2-(pyridin-2-yl)pyrimidine 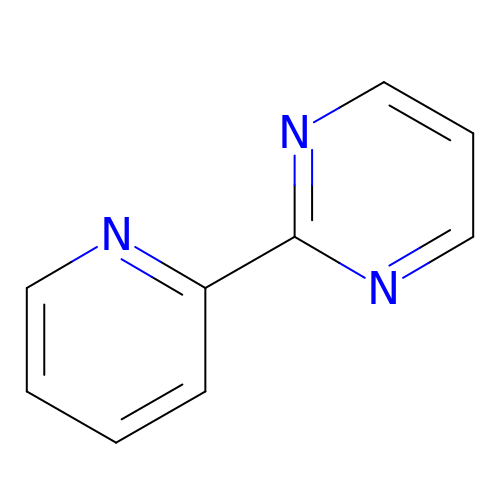| C9 H7 N3 | YJVKLLJCUMQBHN-UHFFFAOYSA-N>[2x]SAPRESPLPYHIPLDPEGSLELSWNVSYTQEAIHFQLLVRRLKAGVLFGMSDRGELENADLVVLWTDGDTAYFADAWSDQKGQIHLDPQQDYQLLQVQRTPEGLTLLFKRPFGTCDPKDYLIEDGTVHLVYGILEEPFRSLEAINGSGLQMGLQRVQLLKPNIPEPELPSDACTMEVQAPNIQIPSQETTYWCYIKELPKGFSRHHIIKYEPIVTKGNEALVHHMEVFQCAPEMDSVPHFSGPCDSKMKPDRLNYCRHVLAAWALGAKAFYYPEEAGLAFGGPGSSRYLRLEVHYHNPLVIEGRNDSSGIRLYYTAKLRRFNAGIMELGLVYTPVMAIPPRETAFILTGYCTDKCTQLALPPSGIHIFASQLHTHLTGRKVVTVLVRDGREWEIVNQDNHYSPHFQEIRMLKKVVSVHPGDVLITSCTYNTEDRELATVGGFGILEEMCVNYVHYYPQTQLELCKSAVDAGFLQKYFHLINRFNNEDVCTCPQASVSQQFTSVPWNSFNRDVLKALYSFAPISMHCNKSSAVRFQGEWNLQPLPKVISTLEEPTPQCPTSQGRSPAGPTVVSIGGGKG

Dopamine β-hydroxylase (EC 1.14.17.1, dopamine β-monooxygenase) (DBH) catalyzes the hydroxylation of dopamine to norepinephrine and is thus vital for regulation of these neurotransmitters. DBH is an ascorbate-dependent glycoprotein that requires two type 2 bound copper ions per subunit to be active. Each chain folds into four domains: the DOMON domain, the catalytic CuH and CuM domains, and the C-terminal dimerization domain. The DOMON domain has an immunoglobulin (Ig)–like β-sandwich structure, the catalytic core (the CuH and CuM domains) has the same topology as the structure of PHM, and the dimerization domains consisting of two antiparallel α helices form a four-helix bundle.

Here, we report the first crystal structure of DBH: the structure of full-length dimeric human DBH. In the A chain, the two catalytic CuH and CuM domains are in a closed conformation, and in the B chain, they adopt the same open conformation as seen in PHM. The conformation in chain B is similar to what was observed in the structure of PHM, with a Cu-Cu distance of approximately 14 Å. However, as seen in Fig. 2C, in chain A the two copper ions are close together—approximately 4 to 5 Å in what appears to be a closed active site with a coupled binuclear copper site, as elaborated on below. Three of the four copper sites are not occupied, but the CuM site in chain A is weakly occupied, and a copper has been modeled. Furthermore, the pH in the crystallization condition is approximately 4.2, well below the pKa of the coordinating histidine residues, which therefore will be protonated and not able to coordinate copper. However, we observe that the helices are definitely linked by C528A-C530B and C530A-C528B disulfide bonds. The asymmetry is also reflected in the dimerization domain, where an extra α helix is seen in the A chain. Behind the possible ligand-binding pocket appears to be a metal ion–binding site coordinated by Asp99 OD1, Leu100 O, Ala115 O, and Asp130 OD1/OD2, with Asp114 and Asp126 quite close. On the basis of the presented structure of human DBH, a possible mode of action is that the closed form represents the catalytically active form, and that the open form is catalytically inactive but allows for loading of substrate, release of product, and recycling of the copper redox states.> MLNQSKILTLQAYDPAKVLVFIGGQRVSGFAADTKIVITRNNDNISVHAGVDGEISNALSRDNTGVMTLSLQNTAKWNGYLAQWQRQANVTGLIYLPVQVEGSQGLSLNTIGWIQKQPDLS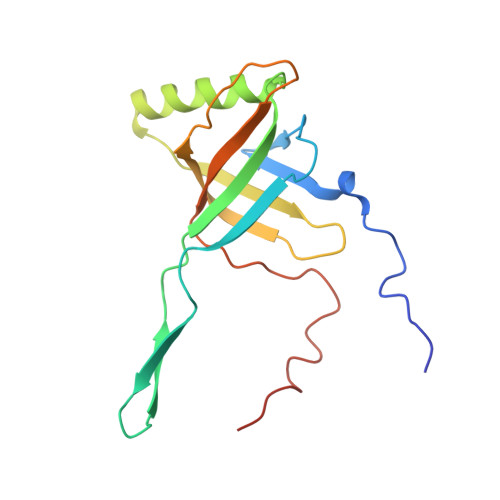YGTEVGQMDWEIGVLDAWLSPDQIQGIAAGITGLLGLDQ> FANFC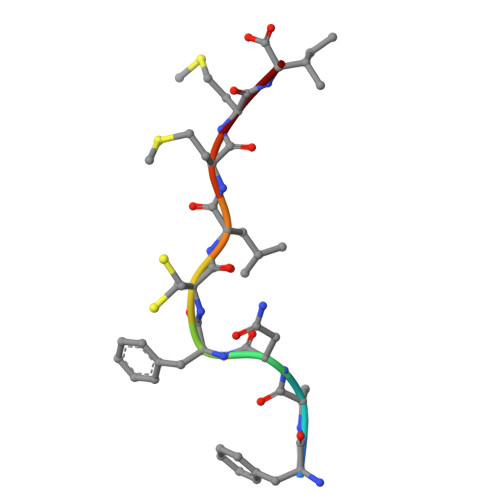LMMI> MEAGITGTWYNQLGSTFIVTAGADGALTGTYVTARGNAESRYVLTGRYDSAPATDGSGTALGWTVAWKNNYRNAHSATTWSGQYVGGAEARINTQWLLTSGTTEENAGYSTLVGHDTFTKVKPSAAS

The long-wavelength beamline I23 at Diamond Light Source overcomes these limitations and extends the accessible wavelength range to λ = 5.9 Å. In this study, we report the determination of diverse protein structures by experimental phasing techniques carried out at long wavelengths on beamline I23 at Diamond Light Source using S, Ca, K, Cl, V, I, Cd, and P as anomalous scatterers. Native-SAD uses light atoms naturally occurring in proteins or bound to proteins. We demonstrate that long-wavelength native-SAD has become a very compelling technique, where a low multiplicity dataset from a single crystal can be sufficient for successful structure determination, making it a general vehicle of choice for experimental phasing.

A second example of a protein without any sulfur atoms is the streptavidin mutant Streptactin XT28. Data were collected at λ = 2.75 Å from crystals that diffracted to better than 1.8 Å resolution. The structure could easily be solved with seven chloride ions bound to the protein although the data was not collected at the chlorine absorption edge (Cl K-edge = 4.39 Å). To the best of our knowledge, this is the first example of Cl-SAD.>MACAAARSPADQDRFICIYPAYLNNKKTIAEGRRIPISKAVENPTATEIQDVCSAVGLNVFLEKNKMYSREWNRDVQYRGRVRVQLKQEDGSLCLVQFPSRKSVMLYAAEMIPKLKTRTQLEHHHHHH[2x];>MGHHHHHHLEILQIIKESQQQHGLRHGDFQRYRGYCSRRQRRLRKTLNFKMGNRHKFTGKKVTEDLLTDNRYLLLVLMDAERAWSYAMQLKQEANTEPRKRFHLLSRLRKAVKHAEELERLCESNRVDAKTKLEAQAYTAYLSGMLRFEHQEWKAAIEAFNKCKTIYEKLASAFTEEQAVLYNQRVEEISPNIRYCAYNIGDQ[2x];>MGSLKVDVEALENSAGATYIRKKGGKVTGDSQPKEQGQGDLKKKKKKKKGKLPKNYDPKVTPDPERWLPMRERSYYRGRKKGKKKDQIGKGTQGATAGASSELDASKTVSSPPTSPRPGSAATVSAST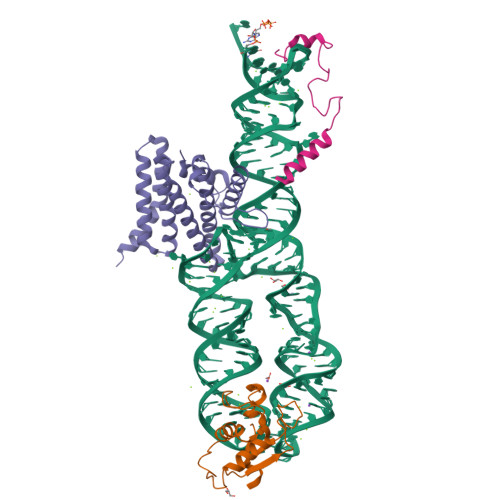SNIIPPRHQKPAGAPATKKKQQQKHHHHHH[2x]>MEIKGESMQKSKFRRICVFCGSSQGKKSSYQDAAVDLGNELVSRNIDLVYGGGSIGLMGLVSQAVHDGGRHVIGIIPKTLMPRELTGETVGEVRAVADMHQRKAEMAKHSDAFIA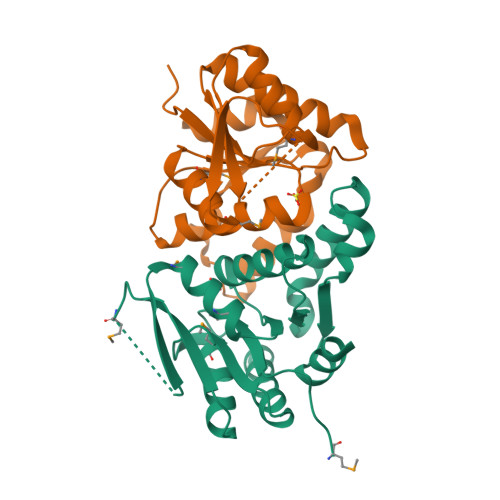LPGGYGTLEELLEVITWAQLGIHDKPVGLLNVDGYYNSLLSFIDKAVEEGFISPTAREIIVSAPTAKELVKKLEEYAPCHERVATKLCWEMERIGYSSEE[2x]>[4x]GAMDD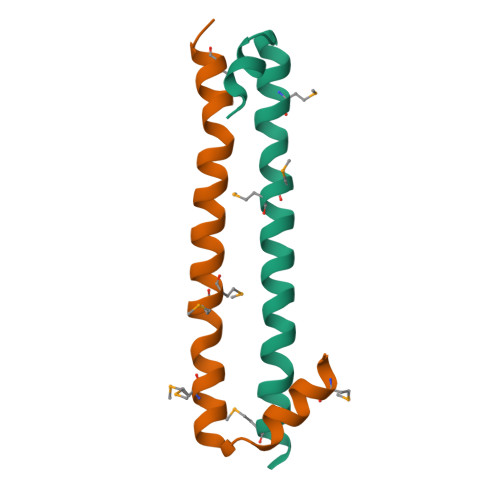FDFLKNLSLEELQMRLKALDPMMEREIEELRQRYTAKRQPILDAMDAK>MNYPAEPFRIKSVETVSMIPRDERLKKMQEAGYNTFLLNSKDIYIDLLTDSGTNAMSDKQWAGMMMGDEAYAGSENFYHLERTVQELFGFKHIVPTHQGRGAENLLSQLAIKPGQYVAGNMYFTTTRYHQEKNGAVFVDIVRDEAHDAGLNIAFKGDIDLKKLQKLIDEKGAENIAYICLAVTVNLAGGQPVSMANMRAVRELTAAHGIKVFYDATRCVENAYFIKEQEQGFENKSIAEIVHEMFSYADGCTMSGKKDCLVNIGGFLCMNDDEMFSSAKELVVVYEGMPSYGGLAGRDMEAMAIGLREAMQYEYIEHRVKQVRYLGDKLKAAGVPIVEPVGGH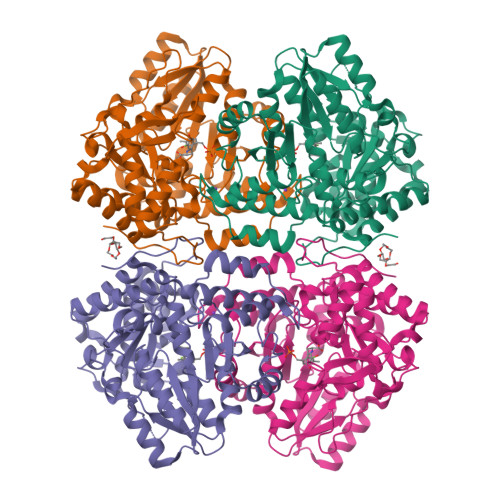AVFLDARRFCEHLTQDEFPAQSLAASIYVETGVRSMERGIISAGRNNVTGEHHRPKLETVRLTIPRRVYTYAHMDVVADGIIKLYQHKEDIRGLKFIYEPKQLRAFTARFDYI[2x]>[3x]MKSQL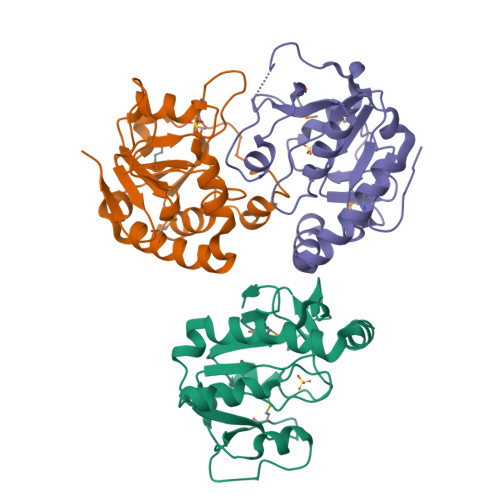RKKTLEALSALSNEDILQKTERMYKYLFSLPEWQNAGTIAVTISRGLEIPTRPVIEQAWEEGKQVCIPKCHPDTKKMQFRTYQTDDQLETVYAGLLEPVIEKTKEVNPSQIDLMIVPGVCFDVNGFRVGFGGGYYDRYLSEYEGKTVSLLLECQLFAHVPRLPHDIPVHKLITEDRIISCFS> QFAKPEDAVKYRQSAATLMASHFGRMTPVVKGQAPYDAAQIKANVEVLKTLSALPWAAFGPGTEGGDARPEIWSDAASFKQKQQAFQDNIVKLSAAADAGDLDKLRAAFGDVGASCKACHDAYRKKK

Cytochromes c′ occur in methanotrophic, denitrifying and photosynthetic bacteria and have proposed roles in protection against nitrosative stress, NO trafficking during denitrification or pathogen defence. All cytochromes c′ have a 4 α-helix bundle structure containing a heme centre with a solvent exposed proximal His ligand and a buried hydrophobic distal pocket with a non-coordinated residue (Leu or Phe, rarely Met or Tyr) in a position to exert steric influence on the binding of diatomic gases. Unusually, cytochromes c′ are able to utilize both heme faces (distal and proximal) as a means of discriminating NO from other diatomic gases. In order to understand the factors controlling distal versus proximal NO coordination, we have examined NO binding to AXCP variants in which the occluding distal residue Leu16 is replaced with residues that are smaller (Ala, Val), of comparable size (Ile) or larger (Phe).

TRIR data for the L16A variant have been described previously. Indeed, recent molecular dynamics simulations of geminate CO-rebinding in wt and L16A AXCP suggest that propionate conformation is a key determinant of distal AXCP-ligand affinity.>MDPVYVDIDADSAFLKALQRAYPMFEVEPRQVTPNDHANARAFSHLAIKLIEQEIDPDSTILDIGSAPARRMMSDRKYHCVCPMRSAEDPERLANYARKLASAAGKVLDRNISGKIGDLQAVMAVPDTETPTFCLHTDVSCRQRADVAIYQDVYAVHAPTSLYHQAIKGVRLAYWVGFDTTPFMYNAMAGAYPSYSTNWADEQVLKAKNIGLCSTDLTEGRRGKLSIMRGKKLEPCDRVLFSVGSTLYPESRKLLKSWHLPSVFHLKGKLSFTCRCDTVVSCEGYVVKRITMSPGLYGKTTGYAVTHHADGFLMCKTTDTVDGERVSFSVCTYVPATICDQMTGILATEVTPEDAQKLLVGLNQRIVVNGRTQRNTNTMKNYMIPVVAQAFSKWAKECRKDMEDEKLLGVRERTLTCCCLWAFKKQKTHTVYKRPDTQSIQKVQAEFDSFVVPSLWSSGLSIPLRTRIKWLLSKVPKTDLTPYSGDAQEARDAEKEAEEEREAELTLEALPPLQAAQEDVQVEIDVEQLEDRAGAAAHHHHHH[12x]

NsP1 is the membrane anchor for the complex, forming dodecameric pores that associate monotopically with the membrane in the necks of the spherules to gate their entrance. Enzymatically, nsP1 also has a role in addition of cap0 structures to the 5′ end of the positive-sense viral RNAs. NsP1 possesses both N′7 methyltransferase and guanylyltransferase activity and reverses the order of these reactions. Each nsP1 protomer is built around a methyltransferase fold common to SAM-dependent methyltransferases with additional insertions (membrane binding and oligomerisation (MBO) loops 1 and 2) and extensions (ring aperture membrane binding oligomerisation (RAMBO) domain) that contribute to pore formation, oligomerization, and membrane binding.

To investigate guanylylation of nsP1, the second step of the reaction, we acquired structures of the protein with SAH and m7GTP in the absence of magnesium, a cofactor necessary for nsP1 GTase activity. As expected, we found that both ligands occupy the active site in a state corresponding to the postmethylation reaction but prior to the m7GMP transfer to the nsP1. However, the definition of the ligand and SAM binding site densities drastically improves, suggesting that the ligands are more stably bound together and that this induces an ordering of the active site. However, there is a slight rotation in the SAH ribose and base, resulting in an ordering of the αC-β4 loop and bringing the side chain of conserved D138 within H-bonding distance of N6 of the SAH base. R92 and R275 of the neighboring protomer move in to directly coordinate the alpha phosphate aligned with H37. This contact provides direct evidence that oligomerization is required to complete the GTP substrate binding site, explaining why nsP1 monomers are inactive for GTase activity. However, it is immediately clear that the substrate is not correctly positioned for nucleophilic attack by the catalytic histidine for guanylylation of the enzyme. Surprisingly, attempts to capture the m7GMP covalently bound intermediate by adding 2 mM MgCl2 and incubating for 2 h yielded exactly the same configuration of the nsP1 active site substrates with two new densities attributable to Mg2+ metal ions. Mg1 appears to coordinate the oxygen atoms from the beta and gamma phosphates (Pβ and Pγ) O2B and O3G, respectively, and a second Mg2 atom appears to coordinate the catalytic H37 and D36 sidechain at 2 Å and 2.3 Å distance. In conclusion, the presence of m7GTP and SAH in the active site results in a metastable conformation that cannot transition directly to the covalent transfer of m7GMP to the catalytic H37, possibly constituting a regulated checkpoint of the capping reaction during infection.>MGKKIIALILIISTAIFGALYMYRNIFSFKDDNNIVALTKGKLISDVYTDKARYYPSDKVTVKIELNNELQEDFRGTIYIFYKHLESIVGKAKIQVNIKSGQKKQLNIFWEAPKDDFKGYLVEVYAVKGNKAIDNKNTAVDVSSDWSKFPRYGYIANFPEQSKEKSALIIEDLNKYHLNGLLFYDWQYKHNKPLAGTVENPDPKWKDIANRDIYGQTVKDYIELAHSKNIMVANYNLMYGGYFDYVKDGAKPEWGLYKDPNHEEQDNHPLPHTWATDRLYLFNPANKDWQNYIFNAEKDAFRVYNFDVWHVGTLGPRGMVYDYNGNPVELSFTYADFLNNAKNALGKRIVCNTVNEYGLINVASGADVDFLYVEIWPPARAHYNFLKQTVDNGYNYSDGKKATVVAAYMNYGIADRSAEFNKHSVRLTDAAIFAAGGDHIELGDTGMLSKEYFPSANLKMSESLVKAMRNYYDFLTAYENLLRDGLKESDNKIEIPGIEISNNGSARTVWTYAKQKDGYDVIHMINLLGIEVSNWRDDLGNYSAPPIIKDFKVKYYLEN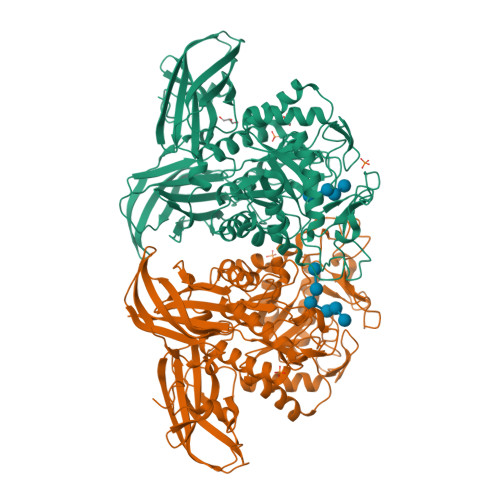DNIKNVYLASPDINDGKVMKLQFKKKEDSKGKYLEISVPELQYWDMIFIKKLEHHHHHH[2x]Citrullination, the loss of a positive charge on the arginine side chain to form citrulline, is catalyzed by peptidylarginine deiminase 4 (PAD4) of the PAD enzyme family. PAD4 is implicated in rheumatoid arthritis (RA), where citrullinated epitopes serve as important diagnostic and pathological factors. The active form of PAD4 is a homodimer, and dimerization greatly affects enzyme activity because monomeric mutants are less active. In this study, we identified GAGs as physiological allosteric coactivators of PAD4.

To explain the lower activatory potential of shorter oligomers, we determined the structure of PAD4 with Dp12 in the absence of calcium. This structure also contained two face-to-back dimers of PAD4, similar to the Dp20-bound structure, but they were connected by a single Dp12 and angled differently (approximately 73° in the x–y plane and approximately 38° in the z–x plane). The Dp12 oligomer was again bound proximal to the region spanning a loop including R123 to R137 of the bottom dimer. In addition, one more Dp12 molecule could reside in loop R123–R137 on the distal side of the top dimer, possibly allowing for the formation of longer PAD4 dimer chains. These structures were observed in the micrographs as a separate 2D class. By plotting the maximum PAD4 activation and Ca0.5 versus (vs) oligomer length, we determined that approximately 12 sugar subunits in the GAG chain are necessary to achieve half of the effects of native heparin. The observed change in the dimer–dimer organization between Dp12 and Dp20 at 0.1 mM Ca2+ consists of the introduction of an additional GAG anchor point for a longer Dp20 oligomer, which introduces torsion sufficient to pull the dimers together and form the 90° double-propeller, cross-like structure.

>MGHHHHHHHHHHHMAQGTLIRVTPEQPTHAVCVLGTLTQLDICSSAPEDCTSFSINASPGVVVDIAHGPPAKKKSTGSSTWPLDPGVEVTLTMKVASGSTGDQKVQISYYGPKTPPVKALLYLTGVEISLCADITRTGKVKPTRAVKDQRTWTWGPCGQGAILLVNCDRDNLESSAMDCEDDEVLDSEDLQDMSLMTLSTKTPKDFFTNHTLVLHVARSEMDKVRVFQATRGKLSSKCSVVLGPKWPSHYLMVPGGKHNMDFYVEALAFPDTDFPGLITLTISLLDTSNLELPEAVVFQDSVVFRVAPWIMTPNTQPPQEVYACSIFENEDFLKSVTTLAMKAKCKLTICPEEENMDDQWMQDEMEIGYIQAPHKTLPVVFDSPRNRGLKEFPIKRVMGPDFGYVTRGPQTGGISGLDSFGNLEVSPPVTVRGKEYPLGRILFGDSCYPSNDSRQMHQALQDFLSAQQVQAPVKLYSDWLSVGHVDEFLSFVPAPDRKGFRLLLASPRSCYKLFQEQQNEGHGEALLFEGIKKKKQQKIKNILSNKTLREHNSFVERCIDWNRELLKRELGLAESDIIDIPQLFKLKEFSKAEAFFPNMVNMLVLGKHLGIPKPFGPVINGRCCLEEKVCSLLEPLGLQCTFINDFFTYHIRHGEVHCGTNVRRKPFSFKWWNMVP[4x]> MNLLQHIAQSRQQLRKSELKVADHVLNDPASVMHSSMAELAHGVGVSEPTIVRFCRAIGCSGFQDLKLKLAQSLAAGASFGQFSIHESDSVADFSLKIFDTTLHSLMEVREHLDTHALERAIAAIAHAQRVEFYGFGASGAVASDAQHKFFRLLLSAAAYSDPHMQAMSAVTLKPSDVAICISQSGRSKDLLITANLVREAGATLITLCPSQTPLADLATVNLAIDVHEDTDIYTPLTSRIAHLVVIDVLAMGVAMARGPDLVN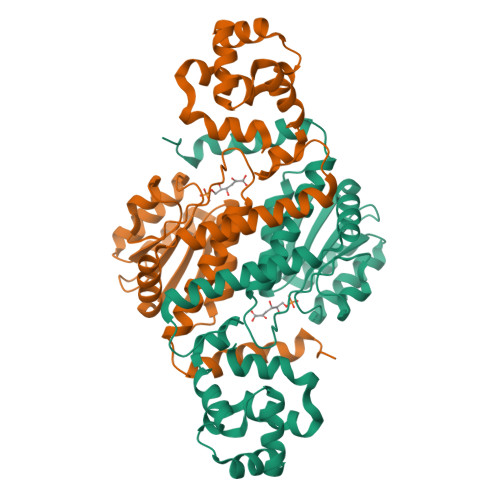HLKSVKRSLRSLRLSPKVMKNQEERGEPS>[8x]GAMDPEFMDGTAAEPRPGAGSLQHAQPPPQPRKKRPEDFKFGKILGEGSFSTVVLARELATSREYAIKILEKRHIIKENKVPYVTRERDVMSRLDHPFFVKLYFCFQDDEKLYFGLSYAKNGELLKYIRKIGSFDETCTRFYTAEIVSALEYLHGKGIIHRDLKPENILLNEDMHIQITDFGTAKVLSPESKQARANSFVGTAQYVSPELLTEKSACKSSDLWALGCIIYQLVAG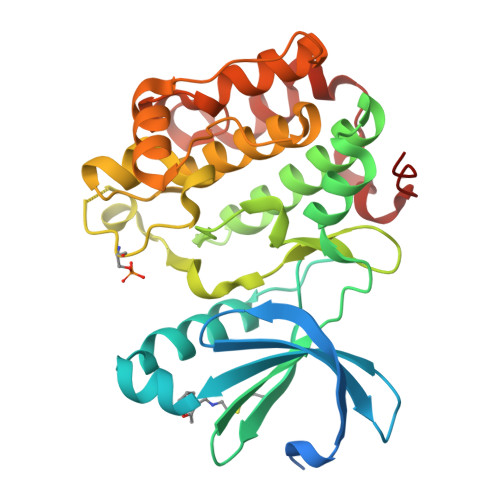LPPFRAGNEYLIFQKIIKLEYDFPEKFFPKARDLVEKLLVLDATKRLGCEEMEGYGPLKAHPFFESVTWENLHQQTPPKLT>[4x]MGSSHHHHHHENLYFQSMASMKTELIRTISLYDTIILHRHVRPDPDAYGSQCGLTEILRETYPEKNIFAVGTPEPSLSFLYSLDEVDNETYEGALVIVCDTANQERIDDQRYPSGAKLMKIDAHPNEDPYGD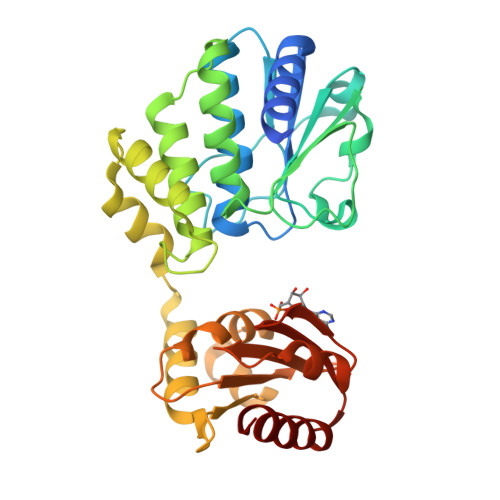LLWVDTSASSVSEMIYELYLEGKEHGWKLNTKAAELIYAGIVGDTGRFLFPNTTEKTLKYAGELIQYPFSSSELFNQLYETKLNVVKLNGFIFQNVSLSENGAASVFIKKDTLEKFGTTASEASQLVGTLGNISGIRAWVFFVEEDDQIRVRFRSKGPVINGLARKYNGGGHPLASGASIYSWDEADRILADLETLCKEHE> MRFYFKFLWLLGIFLIFYFLDFKGSSSYISDRIKNALMNAKNSLLDNVQAYFFQAQNIKEFQKERLILEALKLENADLKERLNSIYPLENPKMTYTPTFMTSFISLEDTHSVSLNPIVNLEENKIYGLVSHNQAIGIAVLEKGRLNGFLNAHKRCAYSVMIGQNQVLGFIGTNFKQELVVDFIVPS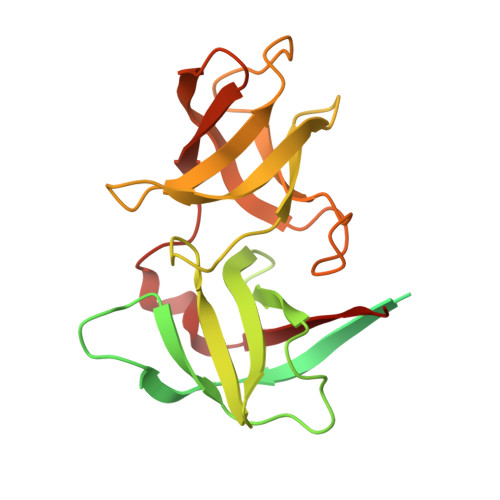AEINIGDQVLTSGLDGIFGAGVFVGEVSSIEDHYTYKSAVLKNAFLSGAKLLRHVFLSDVKN>MIQEHRYDVVIVGAGGAGMRAAVEAGPRARTAVLTKLYPTRSHTGAAQGGMCAALANVEEDNWEWHTFDTVKGGDYLADQDAVEIMCKEAIDAVLDLEKMGMPFNRTPEGRIDQRRFGGHTRDHGKAPVRRACYAADRTGHMILQTLYQNCVKHDVEFFNEFYALDIALTETPAGPVATGVIAYELATGDIHVFHAKAIVFATGGSGRMYKTTSNAHTLTGDGLGIVFRKGLPLEDMEFHQFHPTGLAGLGILISEAVRGEGGRLLNGEGERFMERYAPTIVDLAPRDIVARSMVLEVLEGRGAGPNKDYVYIDVRHLGEDVLEAKLPDITEFARTYLGVDPVKELVPVYPTCHYVMGGIPTTVNGQVLRDNTNVIPGLYAAGECACVSVHGANRLGTNSLLDINVFGRRAGIAAAEYAQNHNFVDMPENPAEMVVGWVGDILSEHGNERVADIRGALQQSMDNNAAVFRTEETLKQALTDIHALKERYSRITVHDKGKRYNSDLLEAIELGFLLELAEVTVVGALNRKESRGGHAREDYPNRDDTNYMRHTMAYKQGTDLLSDIRLDYKPVVQTRYEPMERKY[3x];>MSAPVIDKPEAGDPELPPVPEGAVMVTLKIARFNPENPDAAGWQSFRVPCLPSDRLLNLLHYVKWYLDGTLTFRRSCAHGVCGSDAMRINGVNRLACKVLMRDMLPKNPNKQLTITIEPIRGLPVEKDLVVNMEPFFDAYRAVKPFLVTSGNPPTKERIQSPTDRARYDDTTKCILCACCTTSCPVYWSEGSYFGPAAIVNAHRFIFDSRDEAAAERLDILNEVDGVWRCRTTFNCTEACPRGIQVTQAIQEVKRALMFAR[3x];>MSTQTEVPAPQPKKTRRRTLYRGDPGMWSWVLHRITGATIFFFLFVHVLDTALVRVSPQAYNEVIETYKTPIVGLMEIGLVAAVLFHALNGIRVILIDFWAKGPRYQRQMLAVIAGLFLVIFIAAVGVIGMHMVERFL[3x];>[3x]MSAPGAGESRLGRPAPVMEREHDRPAALDHPRAPRKPRGIPYFEKYAWLFMRFSGIALVFLALGHLFIMLMWQDGVYRIDFNYVAERWASPFWQIWDMALLWLAMIHGANGMRTIIGDYARKNVTKFWLNSLLLLATGFTLVLGSYVLVTFDANISHHHHHHHHHH;>MVLFFEILLVAAVLVITWFAVYALYRLVTDES[3x]

Complex II is both a functional member of the oxidative phosphorylation pathway and the Krebs cycle, thus linking these two energy-harvesting processes. Members of the complex II superfamily are identified as succinate:quinone oxidoreductases (SQRs; or succinate dehydrogenases, SDHs) or quinol:fumarate oxidoreductases (QFRs; or fumarate reductases, FRDs) according to the preferred direction of reaction. No matter the direction, SQRs and QFRs share a common architecture with a large soluble domain and a smaller integral-membrane domain. They are comprised of a soluble flavin-containing subunit, an iron-sulfur cluster-containing subunit, either one or two transmembrane subunits and either zero, one, or two b-type heme groups. Diheme-containing SQRs generally perform menaquinone-linked succinate oxidation, a thermodynamically unfavorable reaction.

In the present study, we obtained a 2.8 Å cryo-electron microscopy (cryo-EM) structure of a trimeric form of an Sdh2 protein from M. smegmatis, which will help us to understand the mechanism of this catalytic process in the diheme-containing SQRs. The dimensions of the Sdh2 trimer are 110 Å in width and 105 Å in height, adopting a mushroom-like shape. Within the trimer, each of the three assemblies contains four canonical proteins: an FAD (flavin adenine dinucleotide)-binding protein (SdhA), an iron-sulfur protein (SdhB), and two membrane-anchored proteins (SdhC and SdhD), each with three transmembrane helices. Here, we have identified a 3 kDa subunit SdhF, which has only one transmembrane helix for its secondary structure, which is located near the transmembrane helix I of SdhC. However, the equivalent QP-binding pocket in M. smegmatis Sdh2 structure is completely blocked by the SdhF subunit, making this site totally inaccessible from the outside. Two b-type hemes, denoted as bP heme and bD heme based on their proximity to the hydrophilic subunits, are located in the membrane-spanning regions of the subunits SdhC and SdhD, and their axial ligands are His D107–His C87 and His D65–His C47, respectively. Fifteen phospholipid molecules and six menaquinone/menaquinols are all clearly observed in the structure, which is in agreement with MS. In the present structure, cardiolipin (CL), phosphatidylethanolamine (PE), phosphatidylinositol (PI), and phosphatidic acid (PA) molecules are mainly distributed in the cleft in the transmembrane space formed by neighboring subunits, playing roles in mediating the interaction of subunits within protomers of the assembly and interactions between neighboring protomers of the assembly. The bound MK/MKH2 interacts with the side chains of Gln-D94, Ile-D95, Met-D98, Trp-D102, and Leu-D103 of transmembrane helix V in one protomer, and the Val-D142, Ser-D145, Tyr-D146, Val-D149, and Thr-D150 of transmembrane helix VI in an adjacent protomer of the assembly.> VDISTLPRVKVDLVKPPFVHAHDQVAKTGPRVVEFTMTIEEKKLVIDREGTEIHAMTFNGSVPGPLMVVHEN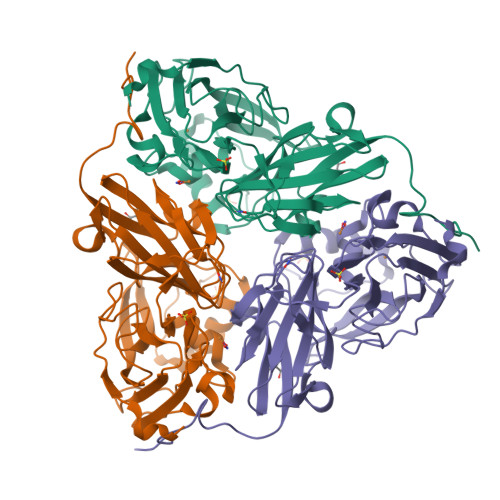DYVELRLINPDTNTLLHNIDFHAATGALGGGALTQVNPGEETTLRFKATKPGVFVYHCAPEGMVPWHVTSGMNGAIMVLPRDGLKDEKGQPLTYDKIYYVGEQDFYVPKDEAGNYKKYETPGEAYEDAVKAMRTLTPTHIVFNGAVGALTGDHALTAAVGERVLVVHSQANRDTRPHLIGGHGDYVWATGKFRNPPDLDQETWLIPGGTAGAAFYTFRQPGVYAYVNHNLIEAFELGAAGHFKVTGEWNDDLMTSVVKPASM>PNGQTKPLPALKLALEYIVPCMNKHGICVVDDFLGKETGQQIGDEVRALHDTGKFTDGQLVSQKSDSSKDIRGDKITWIEGKEPGCETIGLLMSSMDDLIRHCNGKLGSYKINGRTKAMVACYPGNGTGYVRHVDNPNGDGRCVTCIYYLNKDWDAKVSGGILRIFPEGKAQFADIEPKFDRLLFFWSDRRNPHEVQPAYAT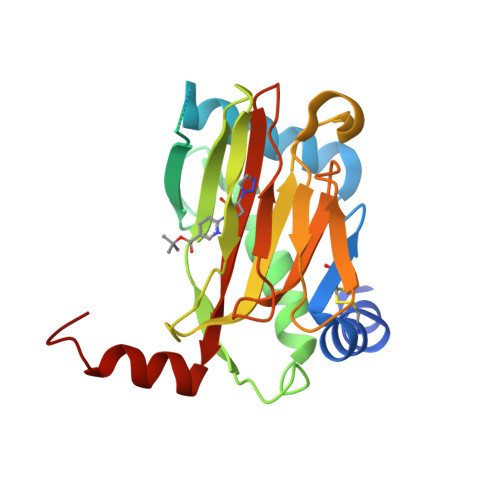RYAITVWYFDADERARAKVKYLTGE[6x]> SM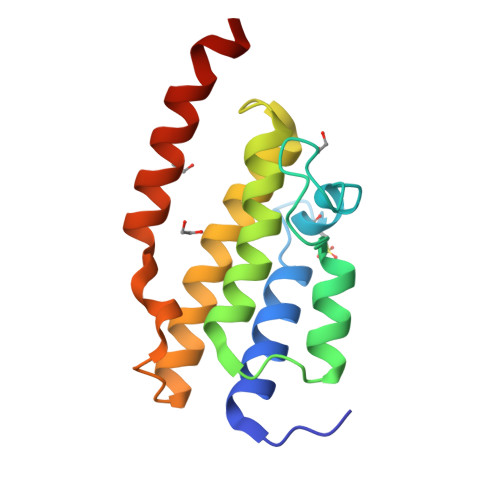NVTLLIQELIHNLFVSVMSHQDDEGRCYSDSLAEIPAVDPNFPNKPPLTFDIIRKNVENNRYRRLDLFQEHMFEVLERARRMNRTDSEIYEDAVELQQFFIKIRDELCKNGEILLSPALSYTTKHLHNDVEKERKEKLPKEIEED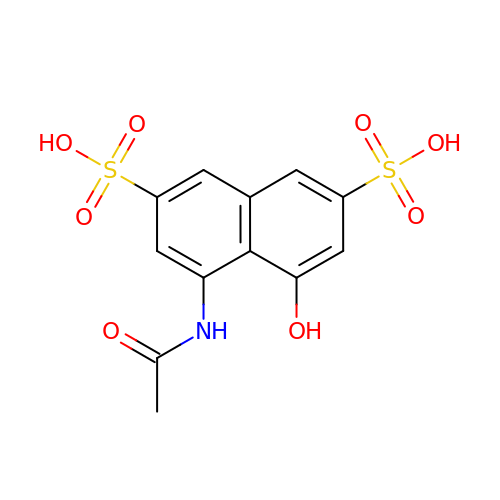4-ACETYLAMINO-5-HYDROXYNAPHTHALENE-2,7-DISULFONIC ACID | C12 H11 N O8 S2 | DACUJXBUANTBKE-UHFFFAOYSA-N>[4x]MRGQGRKESLSDSRDLDGSYDQLTGHPPGPTKKALKQRFLKLLPCCGPQALPSVSETLAAPASLRPHRPRLLDPDSVDDEFELSTVCHRPEGLEQLQEQTKFTRKELQVLYRGFKNECPSGIVNEENFKQIYSQFFPQGDSSTYATFLFNAFDTNHDGSVSFEDFVAGLSVILRGTVDDRLNWAFNLYDLNKDGCITKEEMLDIMKSIYDMMGKYTYPALREEAPREHVESFFQKMDRNKDGVVTIEEFIESCQKDENIMRSMQLFDNVILEGGSSGGHHHHHHHH;>[4x]MAAGVAAWLPFARAAAIGWMPVANCPMPLAPADKNKRQDELIVLNVSGRRFQTWRTTLERYPDTLLGSTEKEFFFNEDTKEYFFDRDPEVFRCVLNFYRTGKLHYPRYECISAYDDELAFYGILPEIIGDCCYEEYKDRKREN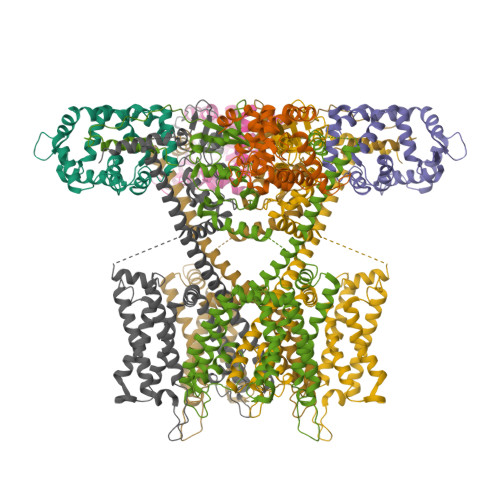AERLMDDNDSENNQESMPSLSFRQTMWRAFENPHTSTLALVFYYVTGFFIAVSVITNVVETVPCGTVPGSKELPCGERYSVAFFCLDTACVMIFTVEYLLRLFAAPSRYRFIRSVMSIIDVVAIMPYYIGLVMTNNEDVSGAFVTLRVFRVFRIFKFSRHSQGLRILGYTLKSCASELGFLLFSLTMAIIIFATVMFYAEKGSSASKFTSIPASFWYTIVTMTTLGYGDMVPKTIAGKIFGSICSLSGVLVIALPVPVIVSNFSRIYHQNQRADKRRAQKKARLARIRVAKTGSSNAYLHSKRNGLLNEALELTGTPEEEHMGKTTSLIESQHHHLLHCLEKTTNHEFIDEQMFEQNCMESSMQNYPSTRSPSLSSHPGLTTTCCSRRSKKTTHLPNSNLPATRLRSMQELSTIHIQGSEQPSLTTSRSSLNLKADDGLRPNCKTSQITTAIISIPTPPALTPEGESRPPPASPGPNTNIPSIASNVVKVSAL>[4x]MSDIKAVAQRALSLMDLTSLTNTETDQEIIDLCRQAKSPAGETAAICIFPRFIPVAKKALKAQQTPHIKIATVTNFPQGNDDLDI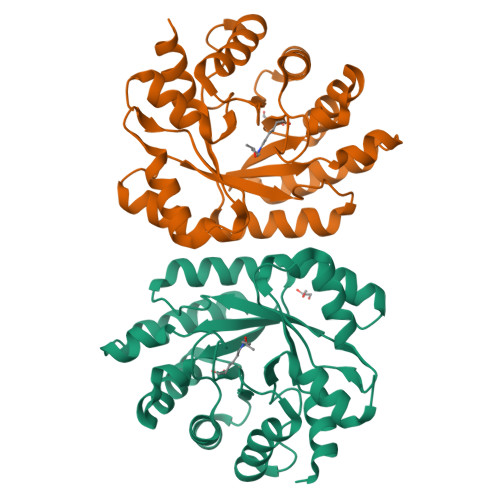ALAETRAAVAYGADEVDLVFPYRALIQGNETIGFDMVKVCKQACSGNAKLKVIIETGELKSEELIRKASEIAINAGADFIKTSTGKVAINATPEAAKVMLTVIKNKNTAVGFKPAGGVRNADDAAIYLDLADNILGNEWADANHFRFGASSLLISLLDTLGHKSNTKSSSNYHHHHHH> MNVTVSIPTILRPHTGGQKSVSASGDTLGAVISDLE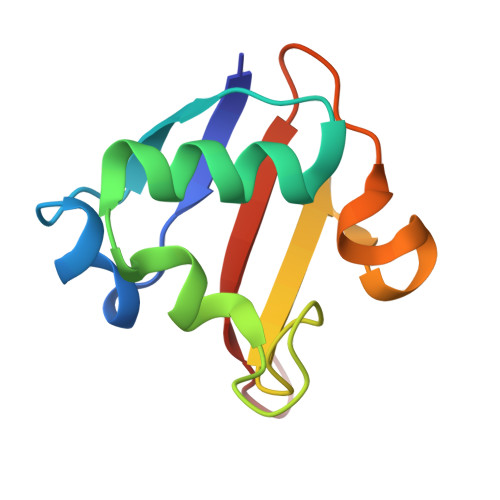ANYSGISERLMDPSSPGKLHRFVNIYVNDEDVRFSGGLATAIADGDSVTILPAVAGG Methylaminomethyl modification of uridine or 2-thiouridine (mnm5U34 or mnm5s2U34) at the wobble position of tRNAs specific for glutamate, lysine and arginine are observed in Escherichia coli and allow for specific recognition of codons ending in A or G. In the biosynthetic pathway responsible for this post-transcriptional modification, the bifunctional enzyme MnmC catalyzes the conversion of its hypermodified substrate carboxymethylaminomethyl uridine (cmnm5U34) to mnm5U34. MnmC (formally known as YfcK or TrmC) is a bifunctional enzyme responsible for the final two steps of biosynthetic pathway of mnm5s2U in tRNAGlu and tRNALys, and mnm5U in tRNAArg. The C-terminal domain (MnmC1) catalyzes the flavin adenine dinucleotide (FAD)-dependent oxidation of the Cα-N bond in cmnm5U34. The resulting imine intermediate is (presumably) non-enzymatically hydrolyzed to 5-aminomethyl uridine (nm5U34), followed by S-adenosyl L-methionine (SAM)-dependent methylation to yield mnm5U in the N-terminal domain active site (MnmC2).

Here we present the FAD/SAM-bound crystal structures of full-length MnmC from E. coli (ecMnmC) and Y. pestis (ypMnmC), and an FAD-bound crystal structure of ypMnmC. In the ecMnmC structure, out of 668 residues, only residues 15–17 and 664–668 could not be modeled. Our structures show that ecMnmC and ypMnmC bind SAM in an almost identical manner. Most interactions between SAM and the protein occur through van der Waals contacts and hydrogen bonds with backbone carbonyl groups, including Phe-67, Thr-69, and Ile-157 in the ecMnmC structure. In addition, the side chains of Phe-24 and Phe-180 contact the nucleoside segment of SAM, shielding it from bulk solvent in the ecMnmC structure, although Phe-24 is not visible due to disorder in ypMnmC structure. The distance between Cϵ of SAM and Oδ of the Asp-178 side chain is 4.1 Å in ecMnmC and 3.6 Å in ypMnmC. The next closest polar side chain belongs to Asp-26 in ecMnmC, which is 6.6 Å away. FAD interacts extensively with the C-terminal ecMnmC1 domain through 16 hydrogen bonds with side chain and backbone atoms of 10 residues within 3.2 Å. Each domain contributes about 40 residues to the interdomain interface, which buries 1578 Å2 of accessible surface area in ecMnmC. In addition, there are three pairs of ionic interactions in ecMnmC; e.g., Arg-94/Glu-637, Arg-107/Glu-375, and Arg-140/Glu-628; only the Arg-140/Glu-640 interaction is present in ypMnmC.

> LGTDDDDKMKHYSIQPANLEFNAEGTPVSRDFDDVYFSNDNGLEETRYVFLGGNQLEVRFPEHPHPLFVVAESGFGTGLNFLTLWQAFDQFREAHPQAQLQRLHFISFEKFPLTRADLALAHQHWPELAPWAEQLQAQWPMPLPGCHRLLLDAGRVTLDLWFGDINELTSQLDDSLNQKVDAWFLDGFAPAKNPDMWTQNLFNAMARLARPGGTLATFTSAGFVRRGLQDAGFTMQKRKGFGRKREMLCGVMEQTLPLPCSAPWFNRTGSSKREAAIIGGGIASALLSLALLRRGWQVTLYCADEAPALGASGNRQGALYPLLSKHDEALNRFFSNAFTFARRFYDQLPVKFDHDWCGVTQLGWDEKSQHKIAQMLSMDLPAELAVAVEANAVEQITGVATNCSGITYPQGGWLCPAELTRNVLELAQQQGLQIYYQYQLQNFSRKDDCWLLNFAGDQQATHSVVVLANGHQISRFSQTSTLPVYSVAGQVSHIPTTPELAELKQVLCYDGYLTPQNPANQHHCIGASYHRGSEDTAYSEDDQQQNRQRLIDCFPQAQWAKEVDVSDKEARCGVRCATRDHLPMVGNVPDYEATLVEYASLAEQKDEAVSAPVFDDLFMFAALGSRGLCSAPLCAEILAAQMSDEPIPMDASTLAALNPNRLWVRKLLKGKAVKAG>[2x]GAMMSRLKTAVYDYLNDVDITECTEMDLLCQLS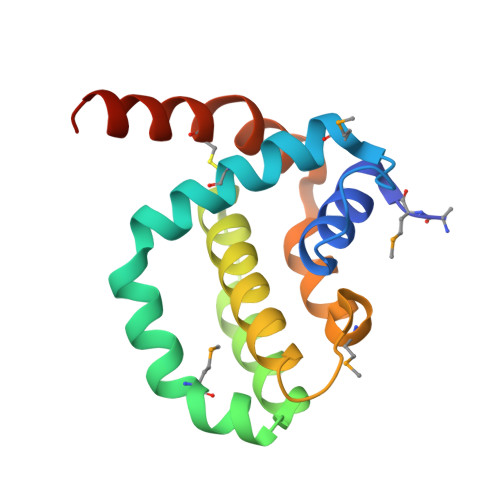NCCDFINETYAKNYDTLYDIMERDILSYNIVNIKNTLTFALRDASPSVKLATLTLLASVIKKLNKIQHTDAAMFSEVIDGIVAEEQQVIGFIQKKCKYNTTYYNVRSGGCK>MSKLTTGSFSIEDLESVQITINNIVGAAKEAAEKAEEELGPMGPTPFPTAATVRDWSFTLFDRYEPVYTPMCDQCCYCTFGPCNLEGNRRGACGLDMKGQAAREFFLRCITGCACHSAHGRHLLDHIISIFGEDMPINMGASNVIAPNIQLITGRQPKTLGDLKPIMEYVEEELGQLLATVHAGQEGAAIDYDNKAMLAGILDHVGMEVSDIAQVTALGFPKSDPEAPLVEVGMGTLDASKPVIIAIGHNVAGVTYIMDYMEDNNLTDKMEIGGLCCTAFDMTRYKREDRKPPYAKIVGTISKELKVVRSGIPDVIVIDEQCVRADLVEEGKKLKIPVIASNEKVMYGLPDRTNDDVDAIIEDIKTGKIPGCVMLDYEKLGELVPRLAMEMAPLREGISAIPSDEEMASLVAKCVACGECALACPEELDIPDAIQAAKEGDFTALDFLHDLCVGCRRCEQVCNKEIPILSVIDKAAQKAIAEEKGLVRAGRGQVSDAEIRAEGLNLVMGTTPGVIAIIGCANYPAGSKDVYRIAEEFLNRNYIVAVSGCSAMDIGMYKDADGKTLYERFPGRFERGNILNTGSCVSNSHISGTCHKVAAIFAGRNLSGNLAEIADYTLNRVGAVGLAWGAYSQKAAAIGTGCNMYGIPAVLGPHSGKYRRALIAKTYDENKWKVYDSRNGSELDIPPSPEFLITTAETWQEACVLLAKNCIRPSDNNMGRSIKLTHWIELSEKYLGVLPEDWWKFVRHEADLPLSRREELLKKLETEHGWEIDWKKKKIISGPKIKFDVSSQPTNLKRLCKEA[2x];>MVDTTKNTKLFTSYGVKTSKAITTEVAAKLISKAKRPLFVVGTGVLDPELLDRAVKIAKAKNIPIAATGSSMPGFVDKDVNAKYINLHQLGFYLTDPDWPGLDGNGNYDTIILLGHKKYYINQVLSAVKNFSDVKSISIDRNYIQNATMSFGNLSKADHIAALDEVIDLL[2x];> MSEFPFEISPMFEGERVRKEGMFVELGGPKSLGLELVRAKPMDEIEDGKVTIVGPDLKDMEEGKTYPWAMIFHVGGELVEPDLESVIERRVHDFINYCQGIMHLNQRYDVWMRISKDTAAKMDSFEPFGKAVMMLFKTELPFIEKMQVTFYTDQAEVEKQMAEAMEIFKARDARTKDLHDEDVDVFYGCTLCQSFAPTNVCVVSPDRVSLCGAINWFDGRAAAKVDPEGPQFAIEKGELLDAKTGEYSGVNEVAKKLSSGEFDKIKLHSFFDAPHTSCGCFEVVGFYIPEVDGIGWVNREYQGMAPNGLGFSTMAGQTGGGKQIVGFLGIGINYFYSPKFIQADGGWNRVVWLPSMLKEKIDEAIPDDMKDKIATEKDVTDIESLKTFLKEKNHPVVANWAAEAEEEEEEEEEEEEVAAEAAPMMMPAAGFQMPAMPAMPMMSGGAGGIKLTFKNAKITIDRMIISEKKEKK

Carbon monoxide dehydrogenase (CODH) and acetyl-CoA synthase (ACS) play major roles in the global carbon cycle through the consumption of CO and CO2 gases, production of acetate, and breakdown of acetate for methane generation. By contrast, methanogenic archaea employ four copies of CODH (α2ε2 heterotetramers) and eight copies of ACS (β monomers) that interact stably with eight copies of CFeSP (γδ heterodimers) to form a massive 2.2 MDa complex called the acetyl-CoA decarbonylase/synthase (ACDS) complex. ACDS plays a central role in that process, wherein the A-cluster of ACS cleaves acetyl-CoA into CO and a methyl moiety, the C-cluster of CODH oxidizes CO to CO2, and the corrinoid of CFeSP receives the methyl moiety, which is reduced to methane in downstream methanogenic metabolism. Through plunge freezing of the ACDS complex, we captured multiple subcomplexes including a CODH tetramer, a CODH/ACS pentamer, and a CODH/ACS hexamer and characterized these subcomplexes via cryogenic electron microscopy (cryo-EM).

With the next-generation chameleon instrument, different dissociation behavior led to formation of (α2ε2)β and (α2ε2)β2 CODH/ACS subcomplexes in addition to the α2ε2 CODH subcomplexes, allowing us to capture methanogenic CODH/ACS subcomplexes. Additionally, from the chameleon-plunged specimen, structures of the MetCODH/ACS pentamer and hexamer were determined, each at a global resolution of 3.2 Å. As expected based on the amino acid sequence, MetACS shares the topology as the A2 and A3 domains of monofunctional and acetogenic ACSs, but lacks the N-terminal A1 domain. The structures reported here reveal that both A2 and A3 of ACS contact CODH. This interface does not bear resemblance to any previously observed CODH/ACS interface; all reported CODH/ACS structures to date are from acetogenic bacteria, wherein it is solely A1 of ACS that interacts with CODH. The MetCODH/ACS interface is also distinct because this interaction includes direct packing of the A-cluster against CODH. In the structure of MetCODH/ACS, we observe density consistent with CO binding to the proximal nickel of the A-cluster. The geometry of Nip is tetrahedral as observed previously for a CO-bound A-cluster. Given that MetACS lacks A1, the ACS packs in more tightly to the CODH compared to the acetogenic CODH/ACS complexes, giving rise to a much shorter distance between the C- and A-clusters, with a measured distance of ~35 Å, and the internal cavity totaling ~50 Å in length. In our structure of MetCODH/ACS, the channel between the C-cluster and A-cluster is open and resembles the open channel near the A-cluster in MoorCODH/ACS.>[2x]MLIAIEGVDGAGKRTLVEKLSGAFRAAGRSVATLAFPRYGQSVAADIAAEALHGEHGDLASSVYAMATLFALDRAGA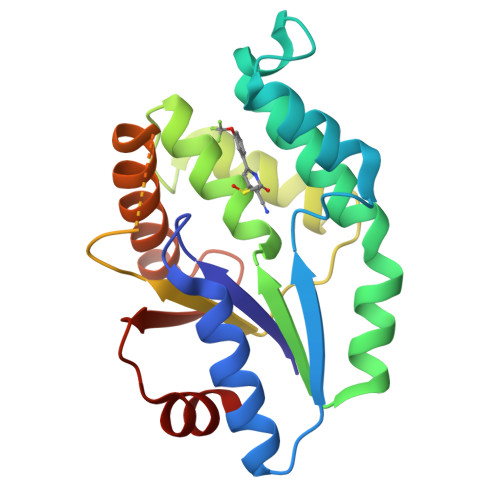VHTIQGLCRGYDVVILDRYVASNAAYSAARLHENAAGKAAAWVQRIEFARLGLPKPDWQVLLAVSAELAGERSRGRAQRDPGRARDNYERDAELQQRTGAVYAELAAQGWGGRWLVVGADVDPGRLAATLAPP ACONITATE 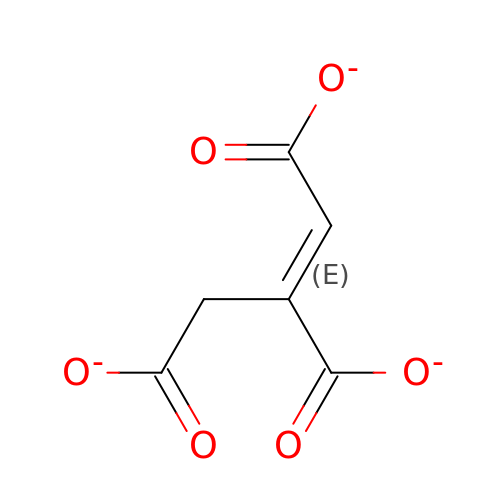ION | C6 H3 O6 | GTZCVFVGUGFEME-HNQUOIGGSA-K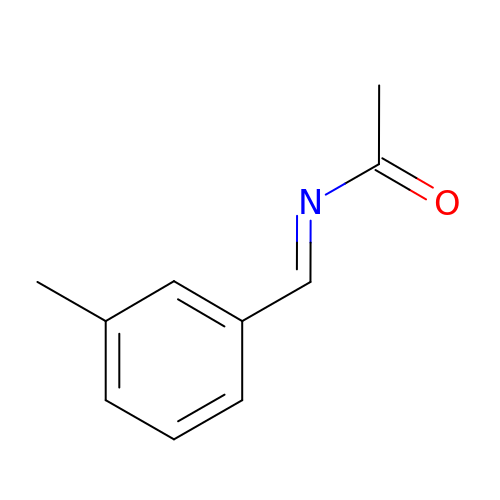N-[(E)-(3-methylphenyl)methylidene]acetamide | C10 H11 N O | KRUUSEWHYKJFLD-YRNVUSSQSA-N> MN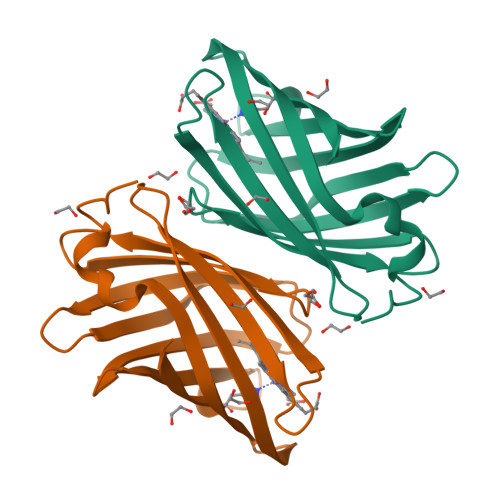QLQQLQNPGESPPVHPFVAPLSYLLGTWRGQGEGEYPTIPSFRYGEEIRFSHSGKPVIAYTQKTWKLESGAPLLAESGYFRPRPDGSIEVVIACSTGLVEVQKGTYNVDEQSIKLKSDLVGNASKVKEISREFELVDGKLSYVVRLSTTTNPLQPHLKAILDKL>GASPSAQELKEQGNRLFVGRKYPEAAACYGRAITRNPLVAVYYTNRALCYLKMQQHEQALADCRRALELDGQSVKAHFFLGQCQLEMESYDEAIANLQRAYSLAKEQRLNFGDDIPSALRIAKKKRWNSIEERR[2x];>XPHEMC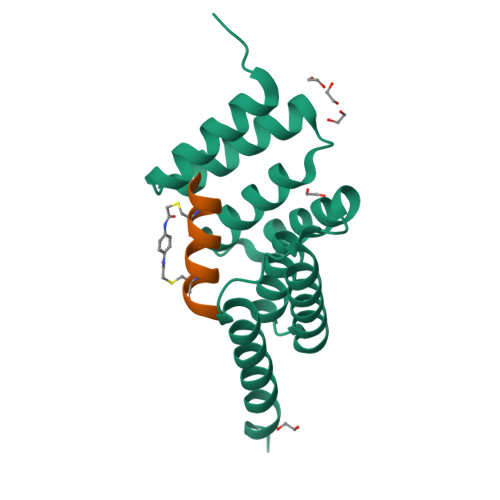YWADAYCRYSX[2x]>[4x]GSGSPLAQQIKNILSLISQADAAGR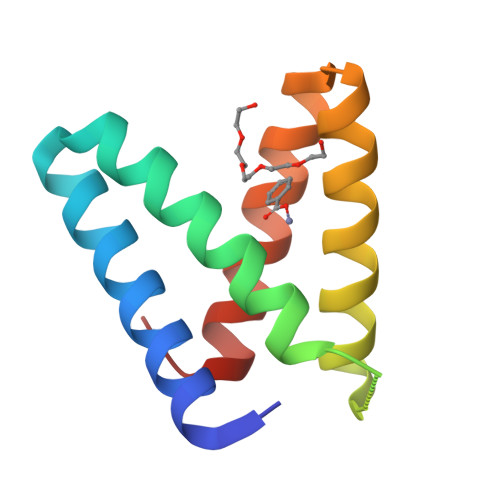MDEVRTLQLNLCQLMVEYFQQSDGDGGSPLAQQIKNIHSFGHQAWAAGRLDEVLTIQENLYQLMKEYFQQSD>PGNDNNNVNNDGVVHVLSKNIDVKNLQGTFYEIATNASDKIFPGLACRCTKYEFSGLKRDGNLGYVLINFSCARNFIFGEKKSEMTFKLILNKPLDENTTTVEEFNASIYLVQGNQQILLNGNINIIYAELNEQNEFEHLILGGQKSIEPMIIMSKYRTVLLDTYNKLINSLYLAGYEPSLLTWPFIIQTD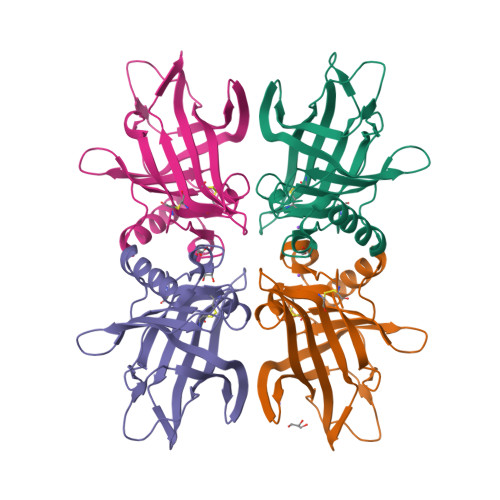QTFCD[4x]> FMVSLPRMVYPQPKVLTPCRKDVLVVTPWLAPIV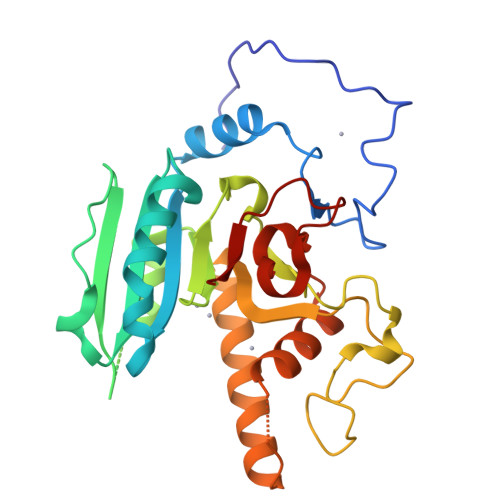WEGTFNIDILNEQFRLQNTTIGLTVFAIKKYVAFLKLFLETAEKHFMVGHRVHYYVFTDQPAAVPRVTLGTGRQLSVLEVRAYKRWQDVSMRRMEMISDFCERRFLSEVDYLVCVDVDMEFRDHVGVEILTPLFGTLHPGFYGSSREAFTYERRPQSQAYIPKDEGDFYYLGGFFGGSVQEVQRLTRACHQAMMVDQANGIEAVWHDASHLNKYLLRHKPTKVLSPEYLWDQQLLGWPAVLRKLRFTAVP> LIPNISPDSFTVAASTGMLSGKSHEMLYDAETGRKISQLDWKIKNVAILKGDISWDPYSFLTLNARGWTSLAS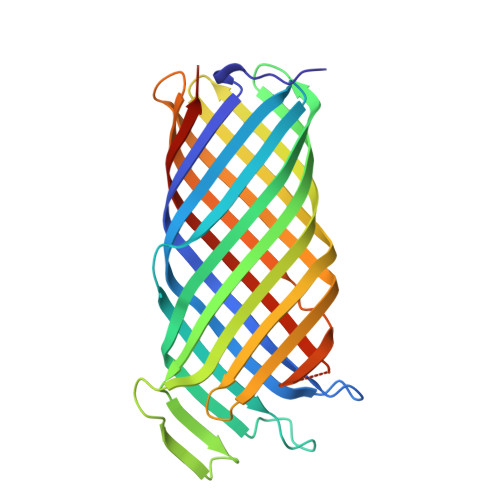GSGNMDNYDWMNENQSEWTDHSSHPATNVNHANEYDLNVKGWLLQDENYKAGITAGYQETRFSWTATGGSYSYNNGAYTGNFPKGVRVIGYNQRFSMPYIGLAGQYRINDFELNALFKFSDWVRAHDNDEHYMRDLTFREKTSGSRYYGTVINAGYYVTPNAKVFAEFTYSKYDEGKGGTQTIDKNSGDSVSIGGDAAGISNKNYTVTAGLQYRFGGGHHHHHH N-(benzylcarbamothioyl)-L-histidine 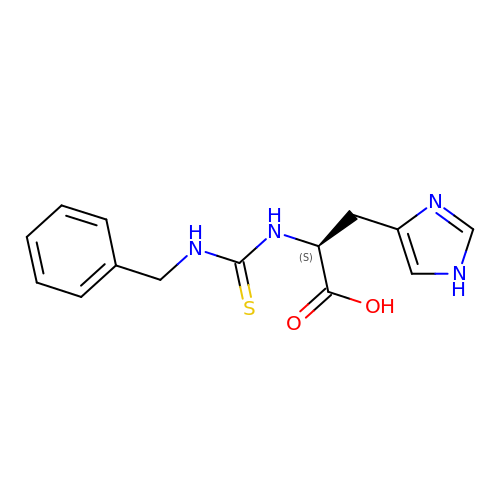| C14 H16 N4 O2 S | VVJPSFQYFNALGR-LBPRGKRZSA-N> MSKQRVFIAGHRGMVGSAIRRQLEQRGDVELVLRTRDELNLLDSRAVHDFFASERIDQVYLAAAKVGGIVANNTYPADFIYQNMMIESNIIHAAHQNDVNKLLFLGSSCIYPKLAKQPMAESELLQGTLEPTNEPYAIAKIAGIKLCESYNRQYGRD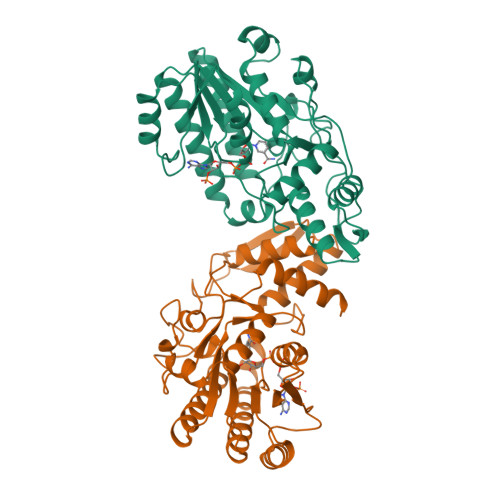YRSVMPTNLYGPHDNFHPSNSHVIPALLRRFHEATAQNAPDVVVWGSGTPMREFLHVDDMAAASIHVMELAHEVWLENTQPMLSHINVGTGVDCTIRDLAQTIAKVVGYKGRVVFDASKPDGTPRKLLDVTRLHQLGWYHEISLEAGLASTYQWFLENQDRFRG> PLGSRYEDAYQYQNIFGPLVKLEADYDKKLKESQTQDNITVRWDLGLNKKRIAYFTLPKTDSDMRLMQGDEICLRYKGDLAPLWKGIGHVIKVPDNYGDEIAIELRSSVGAPVEVTHNFQVDFVWKSTSFDRMQSALKTFAVDETSVSGYIYHKLLGHEVEDVIIKCQLPKRFTAQGLPDLNHSQVYAVKTVLQRPLSLIQGPPGTGKTVTSATIVYHLARQGNGPVLVCAPSNIAVDQLTEKIHQTGLKVVRLCAKSREAIDSPVSFLALHNQIRNMDSMPELQKLQQLKDETGELSSADEKRYRALKRTAERELLMNADVICCTCVGAGDPRLAKMQFRSILIDESTQATEPECMVPVVLGAKQLILVGDHCQLGPVVMCKKAAKAGLSQSLFERLVVLGIRPIRLQVQYRMHPALSAFPSNIFYEGSLQN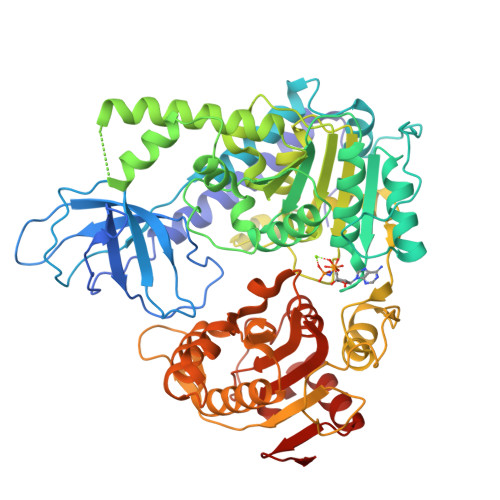GVTAADRVKKGFDFQWPQPDKPMFFYVTQGQEEIASSGTSYLNRTEAANVEKITTKLLKAGAKPDQIGIITPYEGQRSYLVQYMQFSGSLHTKLYQEVEIASVDAFQGREKDFIILSCVRANEHQGIGFLNDPRRLNVALTRARYGVIIVGNPKALSKQPLWNHLLNYYKEQKVLVEGPLNNLRESLMQFS> MKDFTPTPYTLECVATGREFEDTGWMLADPQCKTPSLVRAKYARRQLEVKPDEYGFYKFCDWLPVRRMLKGSSAPVTYKSKGLARHLGLENLYITFNGYYPAIGATMSTCSFKETEAFSVCARAAEDEERVLVVASAGNTARAFAKVCSDNHIKLLLSVPYDNIEALWFEHPLNPCVKLISCEKGGDYFDAIHLSDIALKGPGFYAEGGAKNIARRDGMATTVLSAVTTIGRIPDYYFQAVGSGTGAIAAWEANMRLIEDGRFGSNTMKLMVSQNAPFVPMYDAWQAGSRKMLAYEDDKARRDAEIIDAKVLSNRRPPYGITGGLYDALKATGGEFFVATNAMARKARKLFKELEGVDIYSASGVALASLVNAVAAGKIEKDAVVMLNITGGGEEHFKEDKELWYLKPSHVFPLE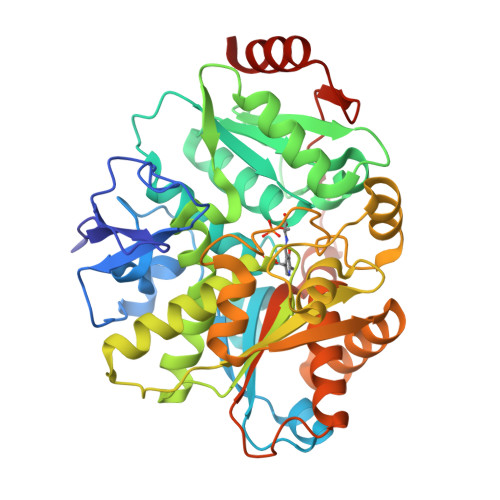PDTDDVVAKVEALFAKNIAE> SAGTSVTLQLDDGSGRTYQLREGSNIIGRGQDAQFRLPDTGVSRRHLEIRWDGQ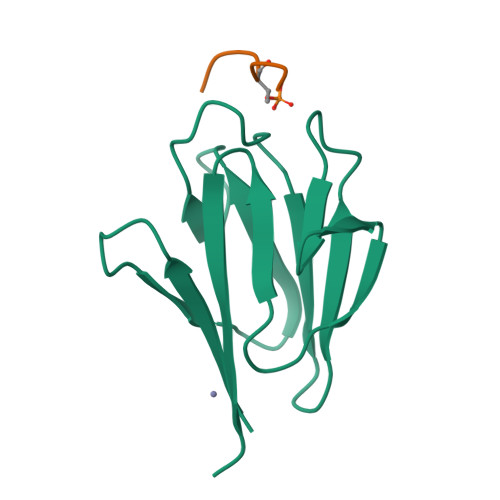VALLADLNSTNGTTVNNAPVQEWQLADGDVIRLGHSEIIVRMHPLT;> DTAPTEKIAYKK> MDKKTIYFISTGNSARSQMAEGWGKEILGEGWNVYSAGIETHGVNPKAIEAMKEVDIDISNHTSDLIDNDIL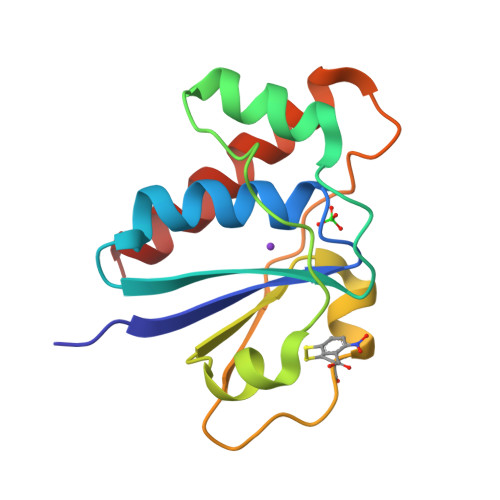KQSDLVVTLSSDADNNCPILPPNVKKEHWGFDDPAGKEWSEFQRVRDEIKLAIEKFKLR> MNARKAPEFPAWPQYDDAERNGLVRALEQGQWWRMGGDEVNSFEREFAAHHGAAHALAVTNGTHALELALQVMGVGPGTEVIVPAFTFISSSQAAQRLGAVTVPVDVDAATYNLDPEAVAAAVTPRTKVIMPVHMAGLMADMDALAKISADTGVPLLQDAAHAHGARWQGKRVGELDSIATFSFQNGKLMTAGEGGAVVFPDGETEKYETAFLRHSCGRPRDDRRYFHKIAGSNMRLNEFSASVLRAQLARLDEQIAVRDERWTLLSRLLGAIDGVVPQGGDVRADRNSHYMAMFRIPGLTEERRNALVDRLVEAGLPAFAAFRAIYRTDAFWELGAPDESVDAIARRCPNTDAISSDCVWLHHRVLLA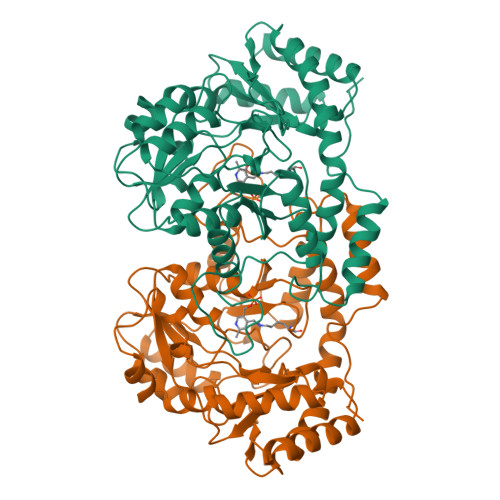GEPELHATAEIIADAVARA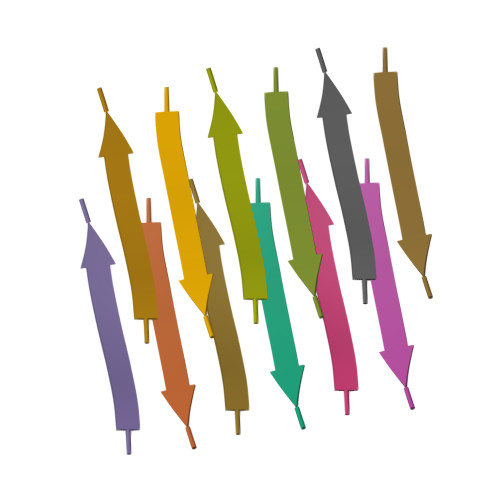>[2x]GGYAGAS> MHHHHHHGGSHHWGGDPERPALGILELSSYARGVKVADAALKAAPVKLLKCEPVEPGRALIMLLGEPEDVAKAMIAALDVAGLGSGNLIDYALIPEIHPQLLPFLKEYKKSEPIKDPNKAIIVAEVSTVAAAIEAADVALRLANVELTSMRLAEHIGGRASFTLIGDKEDVEKAARAIRGVA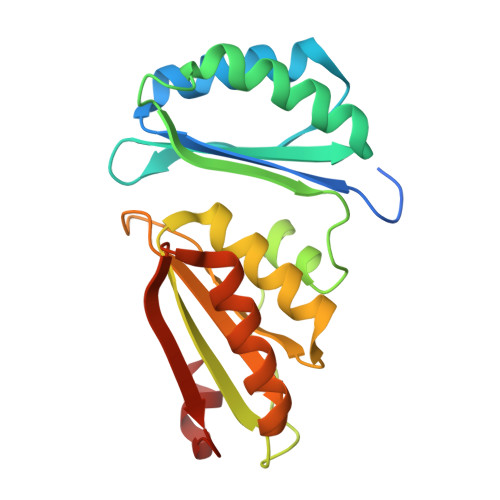GERLLDLEIIEKPVEALIGNEFF>MRGSHHHHHHGSMSETAKKVIVGMSGGVDSSVSAWLLQQQGYQVE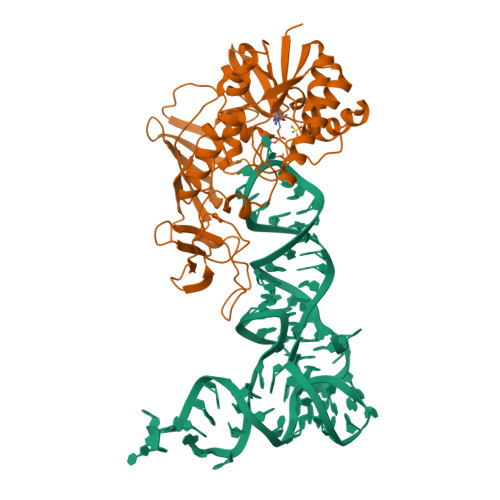GLFMKNWEEDDGEEYCTAAADLADAQAVCDKLGIELHTVNFAAEYWDNVFELFLAEYKAGRTPNPDILCNKEIKFKAFLEFAAEDLGADYIATGHYVRRADVDGKSRLLRGLDSNKDQSYFLYTLSHEQIAQSLFPVGELEKPQVRKIAEDLGLVTAKKKDSTGICFIGERKFREFLGRYLPAQPGKIITVDGDEIGEHQGLMYHTLGQRKGLGIGGTKEGTEEPWYVVDKDVENNILVVAQGHEHPRLMSVGLIAQQLHWVDREPFTGTMRCTVKTRYRQTDIPCTVKALDDDRIEVIFDEPVAAVTPGQSAVFYNGEVCLGGGIIEQRLPLPV[2x]>LTLGNTTSSVILTNYMDTQYYGEIGIGTPPQTFKVVFDTGSSNVWVPSSKCSRLYTACVYHKLFDASDSSSYKHNGTELTLRYSTGTVSGFLSQDIITVGGITVTQMFGEVTEMPALPFMLAEFDGVVGMGFIEQAIGRVTPIFDNIISQGVLKEDVFSFYYNRDS[2x];>[2x]SLGGQIVLGGSDPQHYEGNFHYINLIKTGVWQIQMKGVSVGSSTLLCEDGCLALVDTGASYISGSTSSIEKLMEALGAKKRLFDYVVKCNEGPTLPDISFHLGGKEYTLTSADYVFQESYSSKKLCTLAIHAMDIPPPTGPTWALGATFIRKFYTEFDRRNNRIG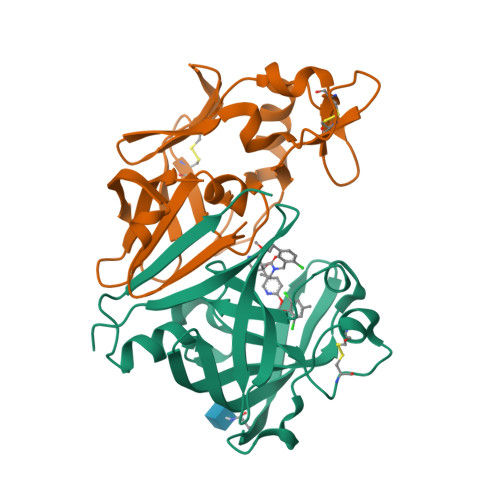FALARHHHHHH>[2x]ALALYTPLPTPTGWTTMGDVAVGDELLGADGKPTRVVAATDVMLGRPCYEVEFSDGTVIVADAAHQWPTSGGIRTSAQLRSGADRIVVAGSAGGYAEQRSATGLLVPVVQIESARRVAS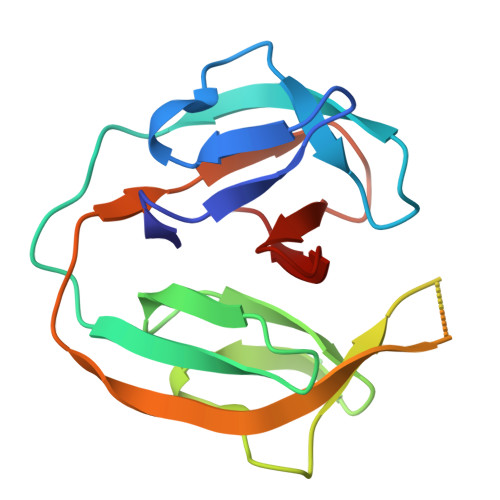VPVRCVEVDNPAHLYLAGRGMVPTHAA>GAMGSPEYLSDEIFSAINNNLPHAYFKNLLFRLVANMD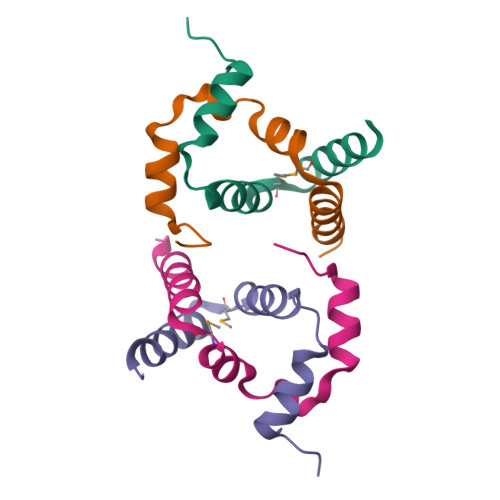RSELSDLGTLIKDNLKRD[4x]>SDGGKVVAATTAQIQEFTKYAGIAATAYCRSVVPGNKWDCVQCQKWVPDGKIITTFTSLLSDTNGYVLRSDKQKTIYLVFRGTNSFRSAITDIVFNFSDYKPVKGAKV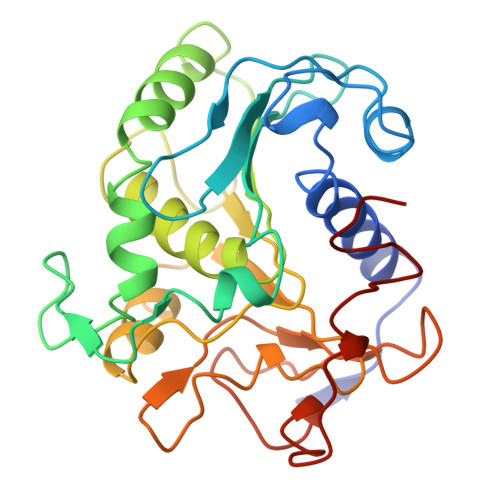HAGFLSSYEQVVNDYFPVVQEQLTAHPTYKVIVTGHSLGGAQALLAGMDLYQREPRLSPKNLSIFTVGGPRVGNPTFAYYVESTGIPFQRTVHKRDIVPHVPPQSFGFLHPGVESWIKSGTSNVQICTSEIETKDCSNSIVPFTSILDHLSYFDINEGSCL[2x]1-(3-MERCAPTO-2-METHYL-PROPIONYL)-PYRROLIDINE-2-CARBOXYLIC 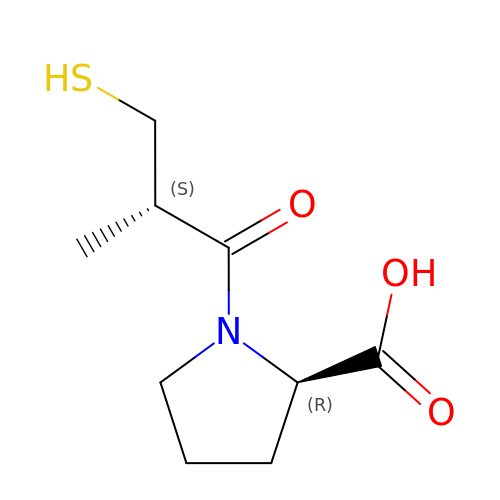ACID | C9 H15 N O3 S | FAKRSMQSSFJEIM-RNFRBKRXSA-N>[2x]GHMADKIKNAKIVFVVGGPGSGKGTQCEKIVAKYGYTHLSSGDLLRAEVASGSERG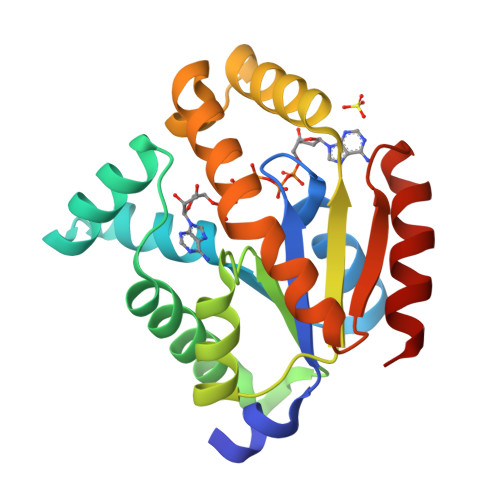KQLQAIMQKGELVPLDTVLDMIKDAMIAKADVSKGYLIDGYPREVKQGEEFEKKIGAPALLLYIDAKGETMVKRLMKRGETSGRADDNEETIKKRLDLYYKATEPVIAFYEQRGIVRKINSELPVDEVFAIVEKAIDELK>MASMTGGQQMGRGSMSRDPLPFFPPLYLGGPEITTENCEREPIHIPGSIQPHGALLTADGHSGEVLQMSLNAATFLGQEPTVLRGQTLAALLPEQWPALQAALPPGCPDALQYRATLDWPAAGHLSLTVHRVGELLILEFEPTEAWDSTGPHALRNAMFALESAPNLRALAEVATQTVRELTGFDRVMLYKFAPDATGEVIAEARREGLHAFLGHRFPASDIPAQARALYTRHLLRLTADTRAAAVPLDPVLNPQTNAPTPLGGAVLRATSPMHMQYLRNMGVGSSLSVSVVVGGQLWGLIACHHQTPYVLPPDLRTTLEYLGRLLSLQVQVKEAADVAAFRQSLREHHARVALAAAHSLSPHDTLSDPALDLLGLMRAGGLILRFEGRWQTLGEVPPAPAVDALLAWLETQPGALVQTDALGQLWPAGADLAPSAAGLLAISVGEGWSECLVWLRPELRLEVAWGGATPDQAKDDLGPRHSFDTYLEEKRGYAEPWHPGEIEEAQDLRDTLTGALGERLSVIRDLNRALTQSNAEWRQYGFVISHHMQEPVRLISQFAELLTRQPRAQDGSPDSPQTERITGFLLRETSRLRSLTQDLHTYTALLSAPPPVRRPTPLGRVVDDVLQDLEPRIADTGASIEVAPELPVIAADAGLLRDLLLHLIGNALTFGGPEPRIAVRTERQGAGWSIAVSDQGAGIAPEYQERIFLLFQRLGSLDEALGNGLGLPLCRKIAELHGGTLTVESAPGEGSTFRCWLPDAGPLPGAADAASSAGGSAGSAGMPERASVPLRLLLVEDNA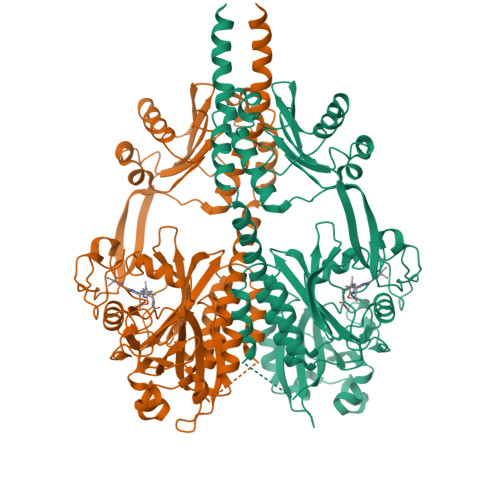ADIFLMEMALEYSSVHTELLVARDGLEALELLEQAKTGGPFPDLILLDLNMPRVDGFELLQALRADPHLAHLPAIVLTTSNDPSDVKRAYALQANSYLTKPSTLEDFLQLIERLTAYWFGTAAIPQTYQPQLEHHHHHH[2x]> MVSDYVPDAGHLVWLNFTPQAGHEQGGRRPALVLSPAAYNGVTGLMQACPVTSRAKGYPFEVTLPAHLGVSGVVLADHCRSLDWRSRRAEQLAEAPADVL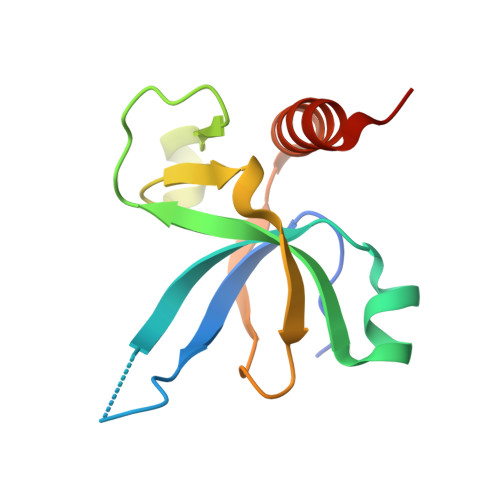AEVRGKLGSLLGMSEKA> SCILPNNNRHQIFNTTQGHYDAVSFIYIPIDGGYMSGSGVVVGENEILTNKHVVNGAKGNPRNISVHPSAKNENDYPNGKFVGQEIIPYPGNSDLAILRVSPNEHNQHIGQVVKPATISSNTDTRINENITVTGY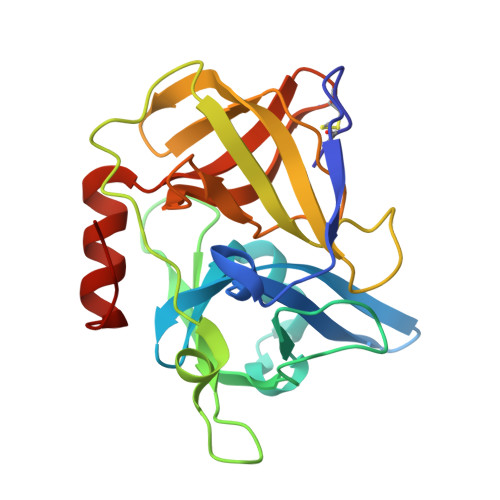PGDKPLATMWESVGKVVYIGGEELRYDLSTVGGNSGSPVFNGKNQVIGIHYGGVCNKYNSSVYINDFVQQFLRNNIPDINIQ>[2x]SNAMKQIIIAIGREFGSGGHLVAKKLAEHYNIPLYSKELLDEVAKDGRYSKEVLERFDEKPMNFAFIPVPAGGTTISLEQDIAIRQFNFIRKKANEEKESFVIVGRCAEEILSDNPNMI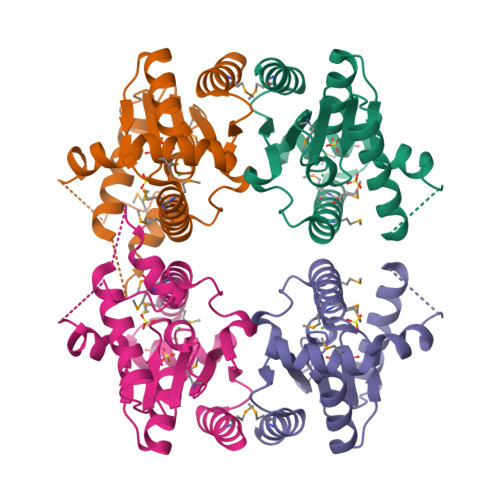SAFILGDKDTKTKRVMEREGVDEKTALNMMKKMDKMRKVYHNFYCESKWGDSRTYDICIKIGKVDVDTATDMIIKYIDSRDN>MDMASRRKNARGLSGAVTALILVIASVIIALVVVGFAFGLFGAFTGQGTVAQVGTATLSASTLTLTVTLKNTGASTQVTGVLINGNSGSVSGMTTISAG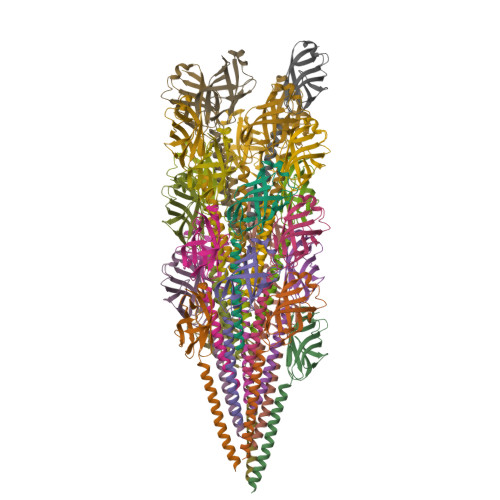VNTYTITISIGSISTTLRGLVGSTISLTLILSNGETVTVSAIVTS[25x]>LQPGIAQQWIQSKREDIVNQMTEACLNQSLDALLSRDLIMKEDYELVSTKPTRTSKVRQLLDTTDIQGEEFAKVIVQKLKDNKQMGLQPYPEILVVSRSPSLNLLQNKSM[10x]

Upon cognate ligand binding, NOD2 oligomerizes and recruits RIP2 via CARD-CARD interactions. Eventually, the NOD2 signalling pathway triggers an inflammatory response through NF-κB, MAPK activation and autophagy as well as the production of anti-bacterial peptides, which protect gut epithelial cells from both residual flora and pathogen invasion. Our biophysical, structural and functional data show that RIP2, via its CARD, can form helical filaments, plausibly nucleated from one end by activated NOD2. Furthermore, we show that RIP2 polymerization is essential for NF-ĸB activation by NOD2, presumably by favouring recruitment of downstream effectors such as the RIP2 ubiquitin ligase XIAP17.

We report the atomic structure of RIP2CARD filaments, solved by high-resolution cryo-electron microscopy (cryo-EM), which reveals the molecular interactions underlying its assembly. Negative-stain and cryo-EM micrographs of samples prepared under the same conditions show that RIP2CARD filaments with bound NOD2CARDSs are shorter, straighter and have a lower tendency to aggregate than RIP2CARD filaments without NOD2. Therefore, the hetero-CARD filaments were used for cryo-EM data collection and analysis. Indexing of the power spectra and symmetry refinement revealed a left-handed helix of 3.56 subunits/turn with an axial rise of 4.848 Å/subunit. The final cryo-EM map at 3.94 Å resolution shows that the filament has an approximate outer diameter of ~75 Å with a central solvent channel of ~25 Å diameter. The crystal structure of RIP2CARD can be unambiguously fitted into the cryo-EM density, with both N- and C-terminal ends orientated towards the outside of the filament. Manual adjustment using the clear density for the α-helices and the larger side chains such as tryptophan and arginine, followed by real space refinement, led to a final atomic model which comprises RIP2CARD residues P433 to Q518. RIP2CARD assembles into a helical arrangement using the conventional type I, II and III interfaces. The cryo-EM structure reveals that the type I and type III interfaces are polar, mediated by interactions of R488 and R444 (type Ia surface) with N457 and D461 (type Ib), and by contacts between E472 and E475 (type IIIa surface) and R483, R488 and T484 (type IIIb). The type II interaction is more hydrophobic for instance involving C455 and M470.> MNIVLMGLPGAGKGTQAEQIIEKYEIPHISTG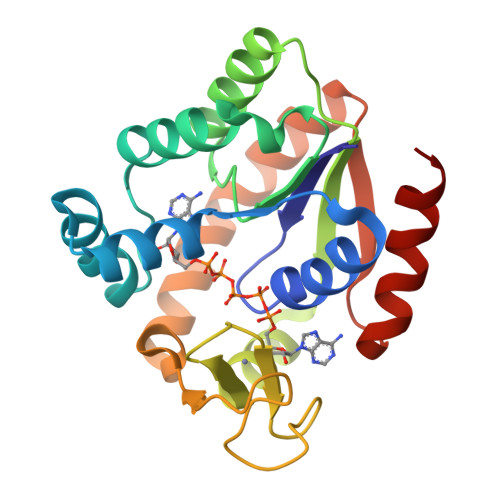DMFRAAIKNGTELGLKAKSFMDQGNLVPDEVTIGIVHERLSKDDCQKGFLLDGFPRTVAQADALDSLLTDLGKKLDYVLNIKVEQEELMKRLTGRWICKTCGATYHTIFNPPAVEGICDKDGGELYQRIDDKPETVKNRLDVNMKQTQPLLDFYSQKGVLKDIDGQQDIKKVFVDINDLLGGLR>MAEIKTSLTFTVRRREPELVVPAEPTPRELKLLSDIDDQEILQSHLAGIQFFRHVPKMRNKKPATVIKEALAKFLVFYYPFAGRVREGPSGKLMVDCSGQGALFIEAEADVTLSQFGDPLQPPFPCVEELLYNVPGTSGIIDTPLLLCQVTHLLCGGFIF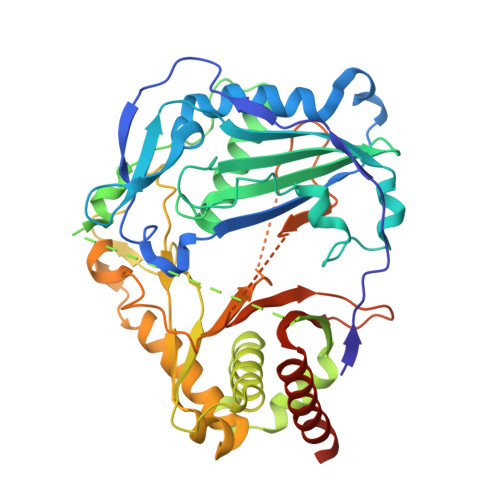AFRFNHTMTDAQGLTLIMSALGEIARGAKAPSILPVWQRELLCSSDRPPMPITHDQIADAAEKDMTQKSFFITNTEISALRRHVPTHLQKCTTFELLTACIWRCHTIALQPDPKEEMHMIWPVNVRNKFKFIPPLPVGYYGNLLAFPDAVSTARDLCNKPLGYALELVMKARYDVTKKRVGSVSDLVKPFKGPVPARHAIVSDLTRSGNNTVDYGWGNPAFVGPASGGIDNNPGLTTYLIPHTNNKGESGIVVPIRLPSGVLDRFVKEINNMLTQAQKNEVLEEHKSPTPSKL[4x]> DFDPV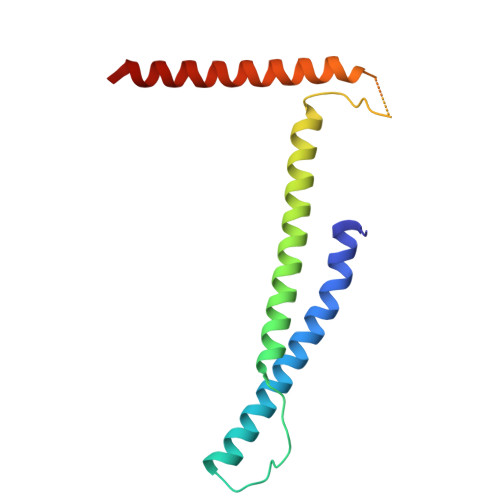QRYKMLIPQLKESLQTLMKVAAQNLIQNTNIDNGQKSSDAPLQRFDKCLEEFYALCDQLELCLRLAHECLSQSCDSAKHSPTLVPTATKPDAVQPDSLPYPQYLAVIKAQITCAKDIHTALLDCANKVT>LGNFSQACYNSAIQGSVLTSTCIRTNGGYNTSSYDLNSVIENVDGSLKWQGSNFIETCRNTQLAGSSELAAECKTRAQQFVSTKINLDDHIAAIDGTLKYELEHHHHHH[2x]

CV-N is a small (11 kDa) natural lectin isolated from cyanobacterium Nostoc ellipsosporum which comprises two quasi-symmetric domains, A (residues 1–38/90–101) and B (residues 39–89 respectively), that are connected to each other by a short helical linker. Functionally, they both bind dimannose, yet the affinity is quite different, with domain B having tighter binding affinity (Kd = 15.3 µM), and domain A showing weak affinity (Kd = 400 µM). To simplify our analyses, we used a designed CV-N variant, P51G-m4, that contains a single high-affinity dimannose binding site (domain B), folds exclusively as a monomer in physiological conditions, and is more stable to thermal denaturation than wild type. Second, we apply our ICDC approach to blindly predict and experimentally validate mutations that allosterically modulate dimannose binding in a natural lectin, cyanovirin-N (CV-N).

We chose position I34, which belongs to category and is 16 Å away from the binding pocket, for experimental validation. I34 exhibits %DFI values lower than 0.2, is at least 16 Å away from binding residues (distal), dynamically coupled and co-evolved with the binding pocket. We found that I34Y binds dimannose with tightest affinity (Kd: 64 µM) of all the mutants tested, a twofold improvement over P51G-m4 (Kd: 117 µM). To glean more information on the mode of binding by I34Y, we determined the X-ray structure of the unbound and dimannose-bound form and compared it with the template protein P51G-m4. The fold is highly conserved as shown by main chain RMSD of 0.16 and 0.20 Å with bound and unbound I34Y, respectively, and tyrosine is well tolerated at position I34. The binding pocket region is also structurally conserved compared to P51G-m4. Analysis of the polar contacts between dimannose and P51G-m4 and I34Y shows an identical number of hydrogen bonds with the ligand, indicating a conserved binding pose. We compared the docked pose of I34Y acquired from Adaptive BP-Dock with the bound X-ray structure. The ligand shows an RMSD value of 0.75 Å. These observations suggest that the increase in binding affinity of I34Y toward dimannose might be mediated by equilibrium dynamics, which are not captured by the crystal structure.Senescence marker protein-30 (SMP30) is a 34-kDa protein whose tissue levels in the liver, kidney, and lung decrease with aging. Biochemical studies suggested that SMP30 is a gluconolactonase (GNL, EC 3.1.1.17) and requires a divalent metal ion such as Zn2+ and Mn2+ for its gluconolactonase activity. In the ascorbic acid biosynthesis pathway, the ring structure of d-glucuronate is cleaved to generate l-gulonate, and then a γ-lactone ring, which is a basic structural framework of ascorbic acid, is formed from l-gulonate by SMP30/GNL. The crystal structure showed that human SMP30/GNL adopts a six-bladed β-propeller fold, which is similar to those of squid diisopropyl-fluorophosphatase (DFPase), drug resistance protein 35 (Drp35), and paraoxonase (PON).

In this study, we determined the crystal structures of mouse SMP30/GNL, which catalyzes formation of the γ-lactone-ring of l-gulonate in the ascorbic acid biosynthetic pathway, in substrate-free and substrate/product-analogue complex forms. The crystal structures of mouse and human SMP30/GNL in the substrate-free form were determined at 1.95 Å and 1.50 Å resolutions, respectively. In the course of the crystallographic refinement, a strong electron density was found inside the β-propeller structure in both mouse and human SMP30/GNL. Since Ca2+ was the most abundant metal ion in the purified sample, a Ca2+ ion was placed at the metal site for the crystallographic refinement. The coordination geometry of the divalent metal ion was quite similar to that of human SMP30/GNL. The asymmetric unit of the mouse and human SMP30/GNL contained two SMP30/GNL molecules. However, molecular weight analysis with static light scattering revealed that mouse and human SMP30/GNL exist as a monomer in solution. The overall structure of mouse SMP30/GNL was essentially the same as that of human SMP30/GNL. Least-squares fitting of mouse and human SMP30/GNL with corresponding 297 Cα atoms gave a root-mean-square (rms) deviation of approximately 0.6 Å. Second, mouse SMP30/GNL has a relatively small substrate-binding cavity.

>[2x]MSSIKVECVLRENYRCGESPVWEEASQSLLFVDIPSKIICRWDTVSNQVQRVAVDAPVSSVALRQLGGYVATIGTKFCALNWENQSVFVLAMVDEDKKNNRFNDGKVDPAGRYFAGTMAEETAPAVLERHQGSLYSLFPDHSVKKYFDQVDISNGLDWSLDHKIFYYIDSLSYTVDAFDYDLQTGQISNRRIVYKMEKDEQIPDGMCIDAEGKLWVACYNGGRVIRLDPETGKRLQTVKLPVDKTTSCCFGGKDYSEMYVTCARDGLNAEGLLRQPDAGNIFKITGLGVKGIAPYSYAG> ETFTVKMGADSGLFQFEPANVTVHPGDTVKWVNNKLPPHNILFDDKQVPGASKELADKLSHSQLMFSPGESYEITFSSDFPAGTYT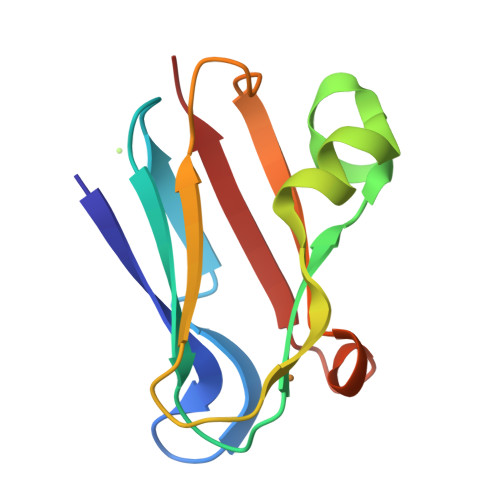YYCAPHRGAGMVGKITVEG RNRs are essential enzymes in all free-living cells, providing the only known de novo pathway for the biosynthesis of deoxyribonucleotides (dNTPs), the immediate precursors for DNA synthesis and repair. Class I RNRs consist of a large, catalytic subunit (α or NrdA), and a smaller, radical-generating subunit (β or NrdB). Additionally, many RNRs possess an overall activity regulation site (a-site) positioned in an N-terminal domain of ~85–100 amino acid residues called the ATP-cone. L. blandensis possesses two RNRs: a class II without ATP-cone, and the class I NrdAi/NrdBi, which lacks an ATP-cone in NrdA and instead contains an ATP-cone positioned at the N-terminus of NrdB.

Binding of dATP to the ATP-cone instead promoted oligomerization of L. blandensis NrdBi to an inactive β4 complex, with a novel tetrameric structure revealed by crystallography. Each monomer consists of an ATP-cone domain (residues 1–103) joined by a short linker (104-106) to a metal-binding α-helical core domain (residues 107–398) and a disordered C-terminus (399-427). The tetrameric arrangement is completely dependent on interactions between the ATP cone domains, as no contacts are made between the core domains in the two dimers that make up the tetramer. The electron density unambiguously confirms the L. blandensis ATP-cone’s ability to bind two molecules of dATP, which it shares with P. aeruginosa NrdA. The two dATP molecules bind in a ‘tail-to-tail’ arrangement that orients the base of the ‘non-canonical’ dATP towards the fourth, most C-terminal helix, an arrangement made possible by the binding of a Mg2+ ion between the triphosphate moieties. The main interactions occur between the last two helices α3 and α4 in respective ATP-cones. A hydrophobic core in L. blandensis NrdB involving residues Met80, Ile92 and Ile93 in both monomers is reinforced by salt bridges between residues Asp73, Asp76 in one monomer and Lys89 in the other. Interestingly, the dATP-induced tetramer leaves free the surfaces of both dimers of L. blandensis NrdB that are thought to interact with the NrdA subunit in productive RNR complexes, which implies that one or two dimers of L. blandensis NrdA could attach to these surfaces in a near-productive fashion in α2β4 or α4β4 complexes. Two metal ions are found to bind to each of the monomers of L. blandensis NrdB. Interestingly, Tyr207 is found near the metal site at the position expected for a radical-carrying Tyr, but it is not hydrogen-bonded to the metal site, its hydroxyl group being at around 6 Å from the side chain of Glu170.

>GSHMSSQEIKKIIKRDYSTAPFVLEKITNAIANAMAALGHGSEQDAKLISMQVYESLLNNKEQESEYIPTVEQVQDMVEDKLMSSEFHDVAKAYIIYRNKRALERKTNIFEKRINLKPYEYPELNEYVAAIRHSYWIHTEFNFTSDIQDFKTGLSEVERSAIKNTMLAISQIEVAVKTFWGDVHHRLPKPEIAAVGATFAESEVRHHDAYSHLLEILGLNEEFKELKKKPVIMKRVHYLETSLKHAKSDDDREYTESILLFALFIEHVSLFSQFLIIMAFNKHKNMLKGISNAVEATSKEEQIHGDFGVDIINIIKKENPEWFDEEHNNLIKEMCLNSFEAESKVVDWIFEKGELDFLPKAVINEFLKNRFNKSLEAIGLEKLFDIDEALLQETEWFDDEIIGTKHGDFFVKRSINYSKRTQSITSDDLF[4x]> MNDSEFHRLADQLWLTIEERLDDWDGDSDIDCEINGGVLTITFENGSKIIINRQ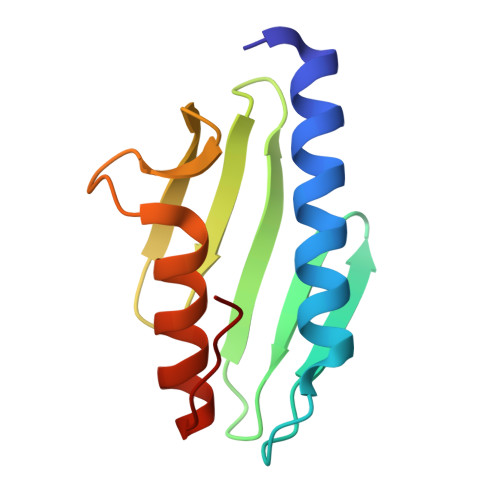EPLHQVWLATKQGGYHFDLKGDEWICDRSGETFWDLLEQAATQQAGETVSFR> MNGIIVDKEKVHPGMPDVVKDAKIALLDAPLEIKKPEFDTNLRIEDPSMIQKFLAQEENMLREMVDKIKSVGANVVITQKGIDDMAQHYLSRAGIYAVRRVKKSDMDKLAKATGASIVSTIDEISSSDLGTAERVEQVKVGE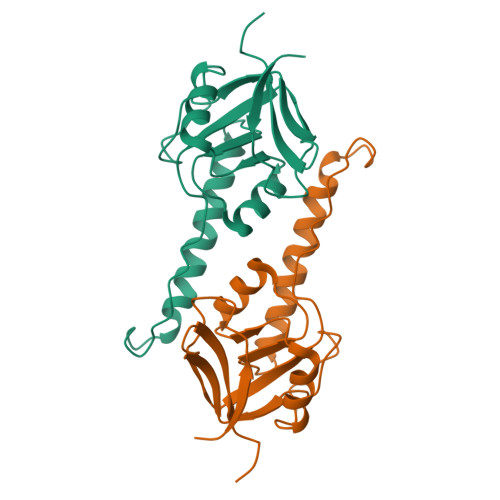DYMTFVTGSKNHHHHHH>MHHHHHHKNITNASILSIVYKDDDLIDLSRYGAEIYNGDKVYYNSIDKNQIRLINLESSTIEVILKKAIVYNSMYENFSTSFWIRIPKYFNSISLNNEYTIINCMENNSGWKVSLNYGEIIWTFQDTQEIKQRVVFKYSQMINISDYINRWIFVTITNNRITKSKIYINGRLIDQKPISNLGNIHASNKIMFKLDGCRDPHRYIVIKYFNLFDKELSEKEIKDLYDNQSNSGILKDFWGDYLQYDKSYYMLNLYDPNKYVDVNNVGIRGYMYLKGPRDNVMTTNIYLNSSLYMGTKFIIKKYASGNKDNIVRNNDRVYINVVVKNKEYRLATNASQAGVEKILSALEIPDVGNLSQVVVMKSKNDQGITNKCKMNLQDNNGNDIGFIGFHQFNNIAKLVASNWYNRQIERSSRTLGCSWEFIPVDDGWRERPL[2x]

Botulinum neurotoxins (BoNT) cause the potentially fatal neuroparalytic disease botulism that arises due to proteolysis of a SNARE protein. Each BoNT is comprised of three domains: a cell binding domain (HC), a translocation domain (HN), and a catalytic (Zn2+ endopeptidase) domain (LC). The HC is responsible for neuronal specificity by targeting both a protein and ganglioside receptor at the neuromuscular junction. Here we present the crystal structures of two BoNT cell binding domains, HC/A4 and HC/A5, in a complex with the oligosaccharide of ganglioside, GD1a and GM1b, respectively.

Consequently, all subsequent analyses below involved molecule A. An initial inspection of the map revealed large positive electron density at the expected GBS, which indicated that GD1a had bound. Monosaccharides Sia5-Gal2 could be modelled with no ambiguity into the electron density and Glc1 partially, but there was insufficient electron density to model Sia6. A total of nine hydrogen bonding interactions were present between HC/A4 and GD1a —there was clear electron density for the two terminal nitrogen atoms of Arg 1282 which interact with Sia5 and Gln 1276. For HC/A4, eight residues form a total of nine hydrogen bonding interactions with the three principal oligosaccharides, GalNAC3, Gal4, and Sia5. Furthermore, HC/A4 displays no water-mediated interactions with the ganglioside, while both HC/A1 and HC/A3 have at least two each. Although there is minimal overall conformational change between HC/A4:GD1a with HC/A4 alone (RMSD of 0.88 Å for all Cα atoms); there is a noticeable change in the relative position of the HCN and HCC subdomains when compared to the unbound structure (RMSD of 0.6 and 0.5 Å, respectively, for all Cα atoms after individual subdomain superimposition). Therefore, upon ganglioside binding, the two subdomains appear to rotate apart like an opening hinge. Inspection of the HC/A4:GD1a GBS residues revealed changes in the relative position of the side chains compared to HC/A4 alone; most notably Arg 1282 (which adopts two conformations in the unbound structure) and Tyr 1123. Upon GD1a binding, these residues shift to form a hydrogen bonding interaction with Sia5. HC/A4 follows this trend as the structure displays a reduction in hydrogen bonding interactions with GD1a and has a reported 1000-fold lower activity in mice.> MWAPPAAIMGDGPTKKVGNQAPLQTQALQTASLRDGPAKRAVWVRHTSSEPQEPTESKAAKERPK;> AARMSEQSICQARAAVMVYDDANKKWVPAGGSTGFSRVHIYHHTGNNTFRVVGRKIQDHQVVINCAIPKGLKYNQATQTFHQWRDARQVYGLNFGSKEDANVFASAMMHALEVLNSQET;>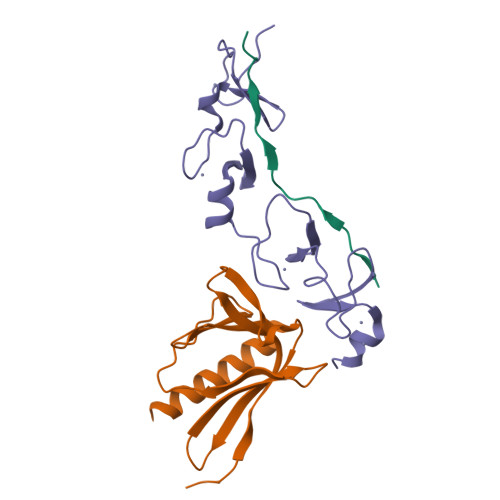 SEKPRCAGCDELIFSNEYTQAENQNWHLKHFCCFDCDSILAGEIYVMVNDKPVCKPCYVKNHAVVCQGCHNAIDPEVQRVTYNNFSWHASTECFLCSCCSKCLIGQKFMPVEGMVFCSVECKKRMS>PGSLNPCIEVVPNITYQCMDQKLSKVPDDIPSSTKNIDLSFNPLKILKSYSFSNFSELQWLDLSRCEIETIEDKAWHGLHHLSNLILTGNPIQSFSPGSFSGLTSLENLVAVETKLASLESFPIGQLITLKKLNVAHNFIHSCKLPAYFSNLTNLVHVDLSYNYIQTITVNDLQFLRENPQVNLSLDMSLNPIDFIQDQAFQGIKLHELTLRGNFNSSNIMKTCLQNLAGLHVHRLILGEFKDERNLEIFEPSIMEGLCDVTIDEFRLTYTNDFSDDIVKFHCLANVSAMSLAGVSIKYLEDVPKHFKWQSLSIIRCQLKQFPTLDLPFLKSLTLTMNKGSISFKKVALPSLSYLDLSRNALSFSGCCSYSDLGTNSLRHLDLSFNGAIIMSANFMGLEELQHLDFQHSTLKRVTEFSAFLSLEKLLYLDISYTNTKIDFDGIFLGLTSLNTLKMAGNSFKDNTLSNVFANTTNLTFLDLSKCQLEQISWGVFDTLHRLQLLNMSHNNLLFLDSSHYNQLYSLSTLDCSFNRIETSKGILQHFPKSLAFFNLTNNSVACICEHQKFLQWVKEQKQFLVNVEQMTCATPVEMNTSLVLDFNNSTCYM[2x];>ESEKQQWFCNSSDAIISYSYCDHLKFPISISSEPCIRLRGTNGFVHVEFIPRGNLKYLYFNLFISVNSIELPKRKEVLCHGHDDDYSFCRALKGETVNTSIPFSFEGILFPKG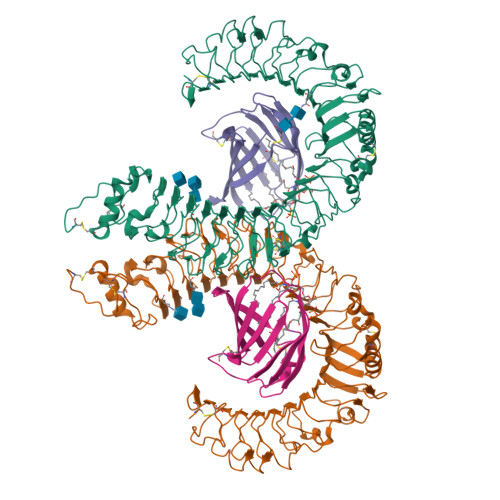HYRCVAEAIAGDTEEKLFCLNFTIIHRRDVN[2x]>MSSSYDEASLAPEETTDSFWEVGNYKRTVKRIDDGHRLCNDLMNCVQERAKIEKAYGQQLTDWAKRWRQLIEKGPQYGSLERAWGAIMTEADKVSELHQEVKNNLLNEDLEKVKNWQKDAYHKQIMGGFKETKEAEDGFRKAQ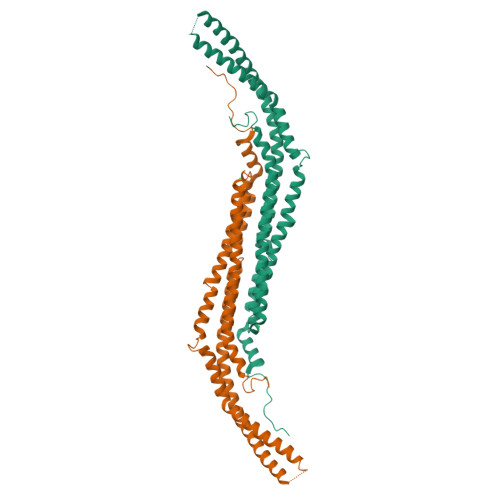KPWAKKMKELEAAKKAYHLACKEEKLAMTREMNSKTEQSVTPEQQKKLQDKVDKCKQDVQKTQEKYEKVLEDVGKTTPQYMENMEQVFEQCQQFEEKRLVFLKEVLLDIKRHLNLAENSSYIHVYRELEQAIRGADAQEDLRWFRSTSGPGMPMNWPQFEEWNPDLPHTTTKKEKQPKKAEG[2x]(4-fluoranyl-3-oxidanyl-phenyl)-[6-(2-fluoranyl-3-oxidanyl-phenyl)pyridin-2-yl]methanone | C18 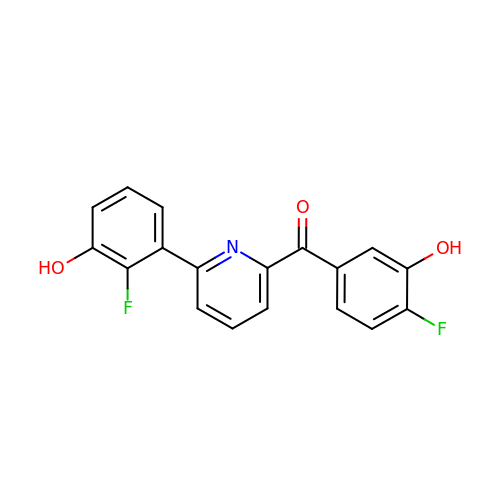H11 F2 N O3 | MXIARVBICPPOCG-UHFFFAOYSA-N>MSSASGLRRGHPAGGEENMTETDAFYKREMFDPAEKYKMDHRRRGIALIFNHERFFWHLTLPERRGTCADRDNLTRRFSDLGFEVKCFNDLKAEELLLKIHEVSTVSHADADCFVCVFLSHGEGNHIYAYDAKIEIQTLTGLFKGDKCHSLVGKPKIFIIQACRGNQHDVPVIPLDVVD[8x];>DAASVYTLPAGADFLMCYSVAEGYYSHRETVNGSWYIQDLCEMLGKYGSSLEFTELLTLVNRKVSQRRVDFCKDPSAIGKK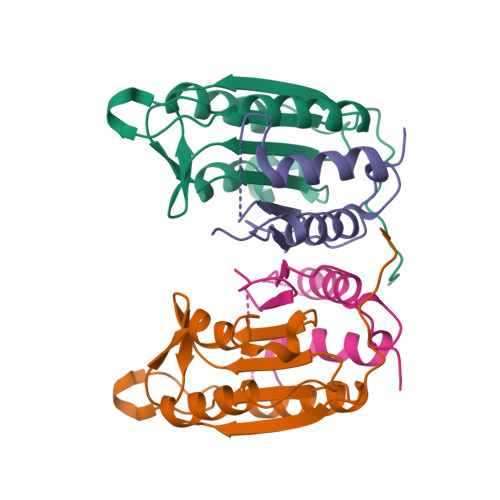QVPCFASMLTKKLHFFPKSNRHHHHHH[8x]>SNAMRKTKTEALKTKEHLMLAALETFYRKGIARTSLNEIAQAAGVTRGALYWHFKNKEDLFDALFQRICDDIENCIAQDAADAEGGSWTVFRHTLLHFFERLQSNDIHYKFHNILFLKCEHTEQNAAVIAIARKHQAIWREKITAVLTEAVENQDLADDLDKETAVIFIKSTLDGLIWRWFSSGESFDLGKTAPRIIGIMMDNLENHPCLRRK[4x]

Transcriptional regulator MtrR inhibits the expression of the multidrug efflux pump operon mtrCDE in the pathogenic bacterium Neisseria gonorrhoeae. A member of the ubiquitous TetR family, MtrR is entirely alpha helical and comprises a helix-turn-helix (HTH) DNA binding motif and a C-terminal ligand binding/dimerization domain. Here, we show that MtrR binds the hormonal steroids progesterone, β-estradiol, and testosterone, which are present at urogenital infection sites, as well as ethinyl estrogen, a component of some hormonal contraceptives. Here, we show that binding of human steroidal hormones results in a comformational change in the MtrR structure rendering it incompatible with DNA binding, thus revealing the structural mechanism of MtrR induction.

The structure of MtrR bound to EST was determined at a resolution of 2.37 Å using de novo phasing by single wavelength anomalous dispersion after selenomethionine substitution of the protein. The stoichiometry of MtrR bound to EST, TES and NDR is 1 ligand:1 protomer. Furthermore, β-estradiol and testosterone are positioned with the five-membered ring pointing towards the dimerization surface whilst progesterone is positioned with the five-membered ring positioned towards the lateral side of the protein. One negatively charged amino acid residue, D171 on helix α8 near the dimerization surface is positioned ~3.4 Å from the hydroxyl group on the five-membered ring of testosterone and estradiol and ~3.8 Å away from the carbonyl on C3 of progesterone. The alignment of MtrR-EST and MtrR-DNA structures reveals three major movements that result in the induction of the protein. The first movement is a 20.8° rotation of the DNA binding domain (α1 through α3), which shifts up and away from the DNA major groove in all MtrR-steroid structures. The second significant movement is a 10° rotation and 4.5 Å shift upward of helix α4. This translation of helix α4 coincides with the upward movement of the HTH domain, away from the DNA, as well as a widening of the ligand binding pocket in the induced form. Last, the flexibility in the loop formed by residues 114–122, between helices α6 and α7, allows a 17.2° outward rotation in helix α7. This movement also aids in the enlargement of the ligand binding pocket as well as a movement of residue W136, which is positioned to obstruct the entrance to the ligand binding pocket in the DNA bound form.> EKLGKLQYSLDYDFQNNQLLVGIIQAAELPALDMGGTSDPYVKVFLLPDKKKKFETKVHRKTLNPVFNEQFTFKVPYSELGGKTLVMAVYDFDRFSKHD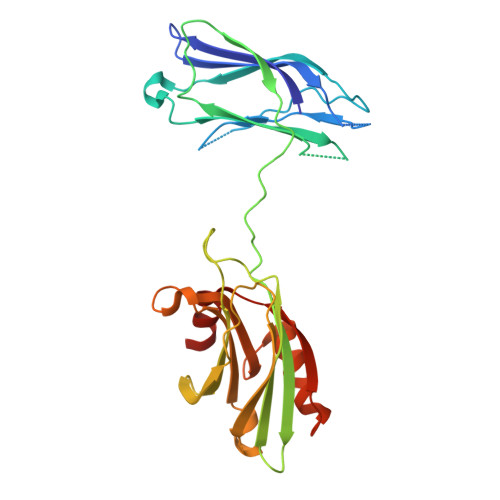IIGEFKVPMNTVDFGHVTEEWRDLQSAEKEEQEKLGDICFSLRYVPTAGKLTVVILEAKNLKKMDVGGLSDPYVKIHLMQNGKRLKKKKTTIKKNTLNPYYNESFSFEVPFEQIQKVQVVVTVLDYDKIGKNDAIGKVFVGYNSTGAELRHWSDMLANPRRPIAQWHTLQVEEEVDAMLAVKK>MKISDGNWLIQPGLNLIHPLQVFEVEQQDNEMVVYAAPRDVRERTWQLDTPLFTLRFFSPQEGIVGVRIEHFQGALNNGPHYPLNILQDVKVTIENTERYAEFKSGNLSARVSKGEFWSLDFLRNGERITGSQVKNNGYVQDTNNQRNYMFERLDLGVGETVYGLGERFTALVRNGQTVETWNRDGGTSTEQAYKNIPFYMTNRGYGVLVNHPQCVSFEVGSEKVSKVQFSVESEYLEYFVIDGPTPKAVLDRYTRFTGRPALPPAWSFGLWLTTSFTTNYDEATVNSFIDGMAERNLPLHVFHFDCFWMKAFQWCDFEWDPLTFPDPEGMIRRLKAKGLKICVWINPYIGQKSPVFKELQEKGYLLKRPDGSLWQWDKWQPGLAIYDFTNPDACKWYADKLKGLVAMGVDCFKTDFGERIPTDVQWFDGSDPQKMHNHYAYIYNELVWNVLKDTVGEEEAVLFARSASVGAQKFPVHWGGDCYANYESMAESLRGGLSIGLSGFGFWSHDIGGFENTAPAHVYKRWCAFGLLSSHSRLHGSKSYRVPWAYDDESCDVVRFFTQLKCRMMPYLYREAARANARGTPMMRAMMMEFPDDPACDYLDRQYMLGDNVMVAPVFTEAGDVQFYLPEGRWTHLWHNDELDGSRW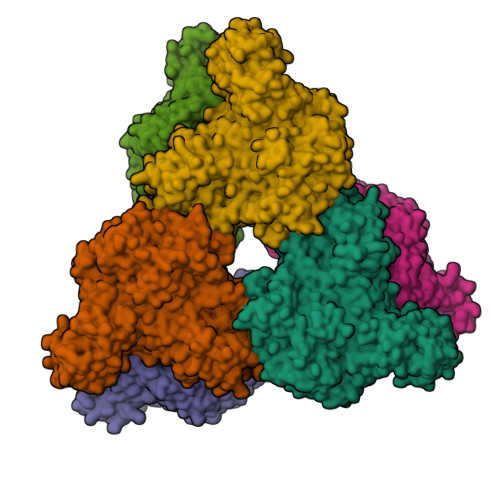HKQQHGFLSLPVYVRDNTLLALGNNDQRPDYVWHEGTAFHLFNLQDGHEAVCEVPAADGSVIFTLKAARTGNTITVTGAGEAKNWTLCLRNVVKVNGLQDGSQAESEQGLVVKPQGNALTITLH[6x]> MEFFGESWKKHLSGEFGKPYFIKLMGFVAEERKHYTVYPPPHQVFTWTQMCDIKDVKVVILGQDPYHGPNQAHGLCFSVQRPVPPPPSLENIYKELSTDIEDFVHPGHGDLSGWAKQGVLLLNAVLTVRAHQANSHKERGWEQFTDAVVSWLNQNSNGLVFLLWGSYAQKKGSAIDRKRHHVLQTAHPSPASVYRG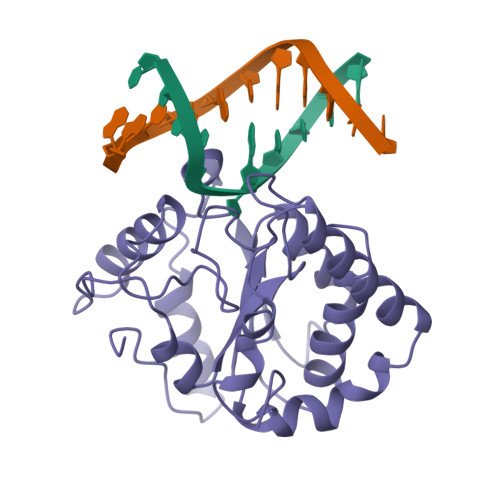FFGCRHFSKTNELLQKSGKKPIDWKEL> EEIILLDYWASMYGMRTRIALEEKKVKYEYREEDLSNKSPLLLQMNPIHKKIPVLIHEGKPICESIIQVQYIDELWPDTNPILPSDPYQRAQARFWADYIDKKTYVPCKALWSESGEKQEAAKIEFIEVLKTLDSELGDKYYFGGNE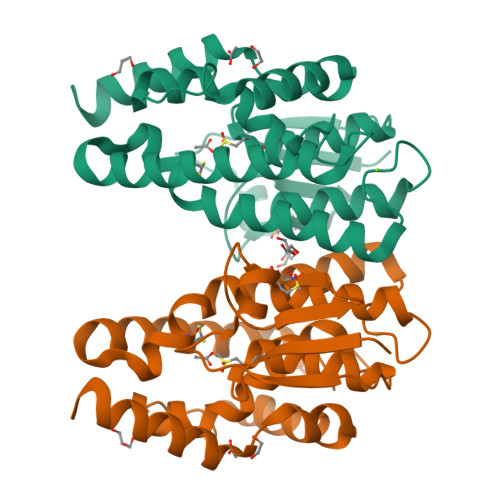FGLVDIAFIGFYSWFRTYEEVANLSIVLEFPKLMAWAQRCLKRESVAKALPDSDKVLKSVSDHRKIILG>MKVISLKKDSFNKGGAVITLLPEDKEDLFTVYQIVDKDDELIFKKKFTSKLDEAGKKKSTDLVKLKIKVISEDFDMKDEYLKYKGVTVTDESGASNVDIPVGKYLSFTLDYVYPFTIIKQNFNKFMQKLLNEACNIEYKSDTAAVVLQEGIAHVCLVTSSSTILKQKIEYSMPKKKRTTDVLKFDEKTEKFYKAIYSAMKKDLNFDKLKTIILCSPGFYAKILMDKIFQYAEEEHNKKILDNKGMFFIAHCSTGYLQGINEVLKNPLYASKLQDTKYSKEIMVMDEFLLHLNKDDDKAWYGEKEVVKAAEYGAISYLLLTDKVLHSDNIAQREEYLKLMDSVESN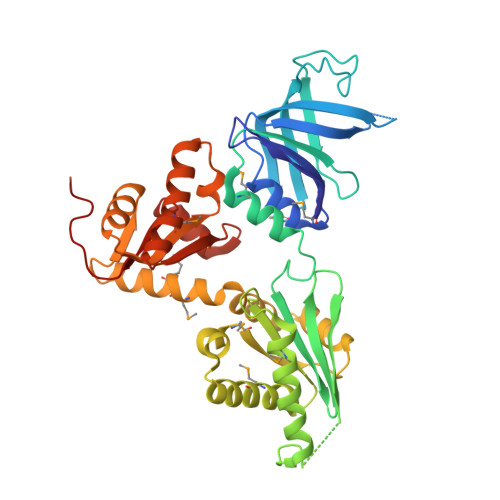GGKALVLSTLHSLGEELDQLTGIACILKYPLPDLDEDDGEE[2x]>MTQRLKDKLAVITGGANGIGRAIAERFAVEGADIAIADLVPAPEAEAAIRNLGRRVLTVKCDVSQPGDVEAFGKQVISTFGRCDILVNNAGIYPLIPFDELTFEQWKKTFEINVDSGFLMAKAFVPGMKRNGWGRIINLTSTTYWLKIEAYTHYISTKAANIGFTRALASDLGKDGITVNAIAPSLVRTATTEASALSAMFDVLPNMLQAIPRLQVPLDLTGA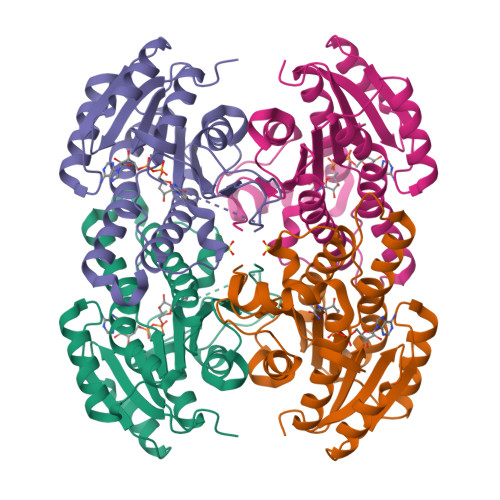AAFLASDDASFITGQTLAVDGGMVRH[2x]> EAQQKTIEAITKAINYMAKRRIGALLTIERDTGMGDYIETGIPLNAKVSSELLINIFIPNTPLHDGAVIMKNNEIAAAACYLPLSESPFISKELGTRHRAAVGISEVTDSLTIIVSEETGGVSVAKNGDLHRELTEEALKEMLEAEFKKNTRD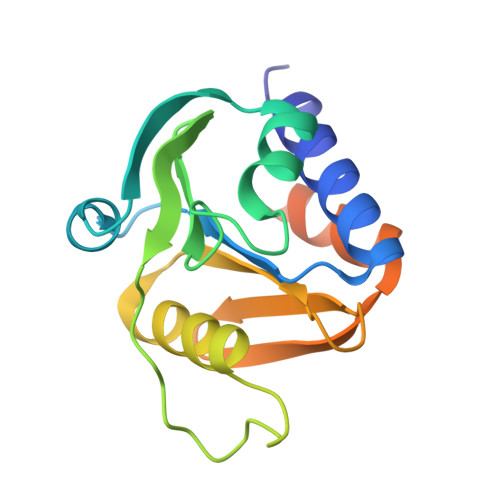TSSNRWYWRGKKNG>[4x]MTWLPLNPIPLKDRVSMIFLQYGQIDVIDGAFVLIDKTGIRTHIPVGSVACIMLEPGTRVSHAAVRLAAQVGTLLVWVGEAGVRVYASGQPGGARSD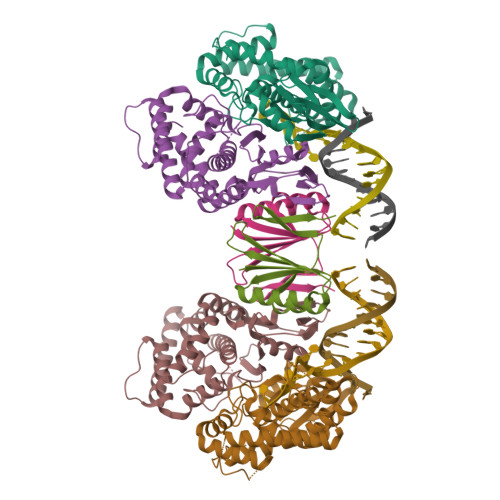KLLYQAKLALDEDLRLKVVRKMFELRFGEPAPARRSVEQLRGIEGSRVRATYALLAKQYGVTWNGRRYDPKDWEKGDTINQCISAATSCLYGVTEAAILAAGYAPAIGFVHTGKPLSFVYDIADIIKFDTVVPKAFEIARRNPGEPDREVRLACRDIFRSSKTLAKLIPLIEDVLAAGEIQPPAPPEDAQPVAIPLPVSLGDAGHRSS;>MSMLVVVTENVPPRLRGRLAIWLLEVRAGVYVGDVSAKIREMIWEQIAGLAEEGNVVMAWATNTETGFEFQTFGLNRRTPVDLDGLRLVSFLPV[2x]(1s,4s)-bicyclo[2.2.1]heptane 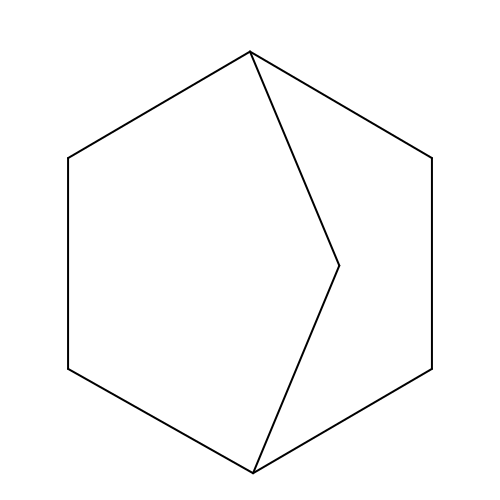| C7 H12 | UMRZSTCPUPJPOJ-KNVOCYPGSA-N>[2x]HHHHHHFNLPPGNYKKPKLLYCSNGGHFLRIAPNGTVDGT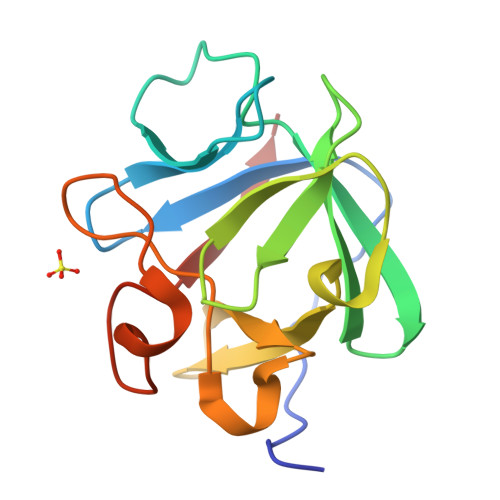RDRSDQHIQLQLSAESVGEVYIKSTETGQYLAMDTDGLLYGSQTPNEECLFLERLEENHYNTYISKKHAEKNWFVGLKKNGSCKRGPRTHYGQKAILFLPLPVSSD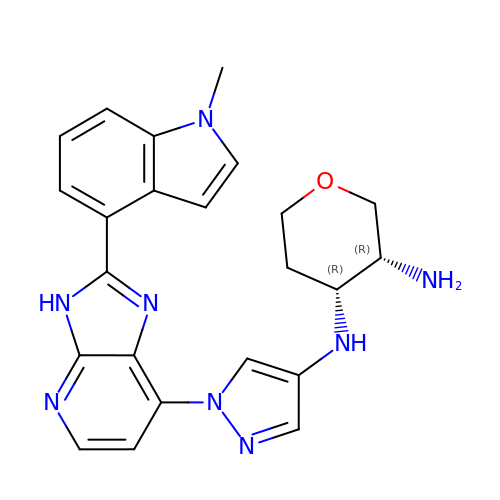(3~{R},4~{R})-~{N}4-[1-[2-(1-methylindol-4-yl)-3~{H}-imidazo[4,5-b]pyridin-7-yl]pyrazol-4-yl]oxane-3,4-diamine | C23 H24 N8 O | MXZJNQSPLXUEQL-ZWKOTPCHSA-N> MTSKTKNIDDIPPEIKEEMIQLYHDLPGIENEYKLIDKIGEGTFSSVYKAKDITGKITKKFASHFWNYGSNYVALKKIYVTSSPQRIYNELNLLYIMTGSSRVAPLCDAKRVRDQVIAVLPYYPHEEFRTFYRDLPIKGIKKYIWELLRALKFVHSKGIIHRDIKPTNFLFNLELGRGVLVDFGLAEAQMDYKSMISSQNDYDNYANTNHDGGYSMRNHEQFCPCIMRNQYSPNSHNQTPPMVTIQNGKVVHLNNVNGVDLTKGYPKNETRRIKRANRAGTRGFRAPEVLMKCGAQST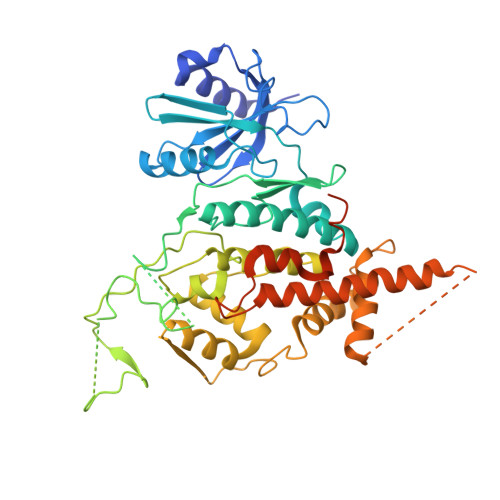KIDIWSVGVILLSLLGRRFPMFQSLDDADSLLELCTIFGWKELRKCAALHGLGFEASGLIWDKPNGYSNGLKEFVYDLLNKECTIGTFPEYSVAFETFGFLQQELHDRMSIEPQLPDPKTNMDAVDAYELKKYQEEIWSDHYWCFQVLEQCFEMDPQKRSSAEDLLKTPFFNELNENTYLLDGESTDEDDVVSSSEADLLDKDVLLISE>MQQEQSYRIEKDFLGEKKIPADAYYGIQTLRATENFPITGYRIHEELIRALAMVKKAAALANMETKRLPAHIGEAIVAACDEIIAGQWHDQFIVDPIQGGAGTSINMNANEVIANRALEIMGKKKGDYFHVRPNSDVNMSQSTNDAFPTAVHIAVLTLLDHLLETMERMRDAFAEKAKAFDPYIKMGRIHLQDAVPIRLGQEFEAYTRVIERDIQRIKQSRGHLYEINMGATAVGTGLNADPRYIESVVKHLREISGYPLVGAENLVDATQNTDAYTEVSAALKVCMMNMSKIANDLRLMASGPRAGLGEITLPARQPGSSIIPGMVCPVMAEVINQIAFQV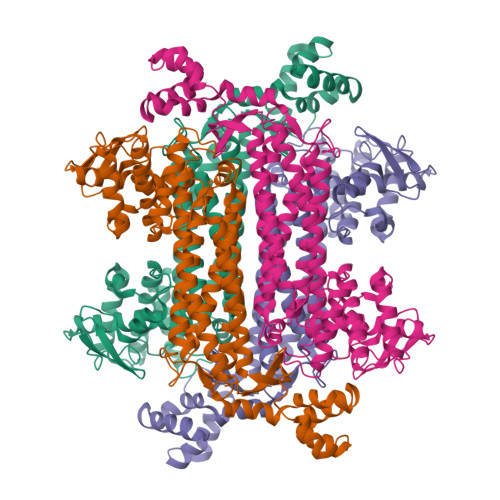IGNDHTICLASEAGQLELNVMEPVLVFNLLQSISIMNNGFRVFTEYCVKGIEANEEKMKEYVEKSVGVITAVNPHIGYEVASRIAREATLTGQSVRDLCRKYDVLSDEELDLILDPYEMTHPGIAGASLLERD[2x]> GHMVSVAAGDKPTNSRQEILEGARRCFAEHGYEGATVRRLEEATGKSR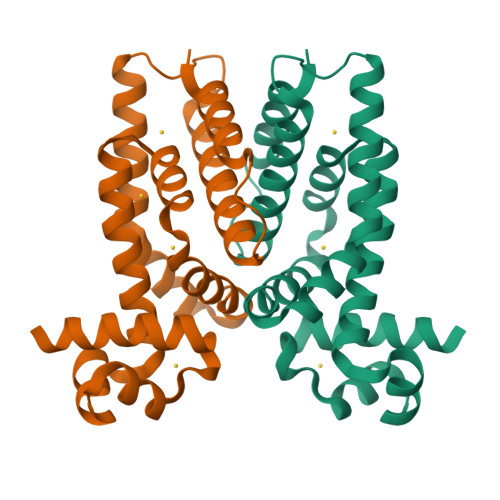GAIFHHFGDKENLFLALAREDAARMAEVVSENGLVEVMRGMLEDPERYDWMSVRLEISKQLRTDPVFRAKWIDHQSVLDEAVRVRLSRNVDKGQMRTDVPIEVLHTFLETVLDGFISRLATGASTEGLSEVLDLVEGTVRKRD2-{4-[3-chloro-2-(2-methoxyphenyl)-1H-indol-5-yl]piperidin-1-yl}-N-methylethanamine | C23 H28 Cl N3 O | 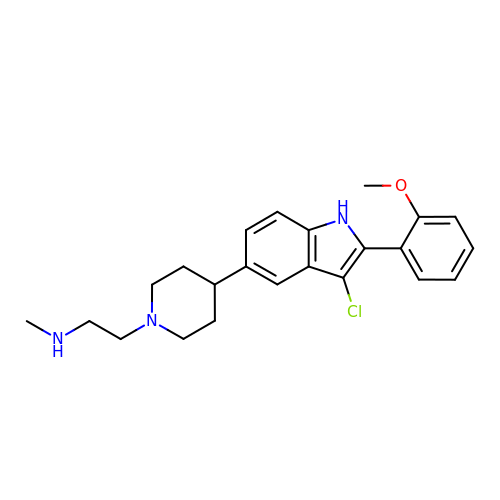SEJLXUYMIRXRMJ-UHFFFAOYSA-N> SRV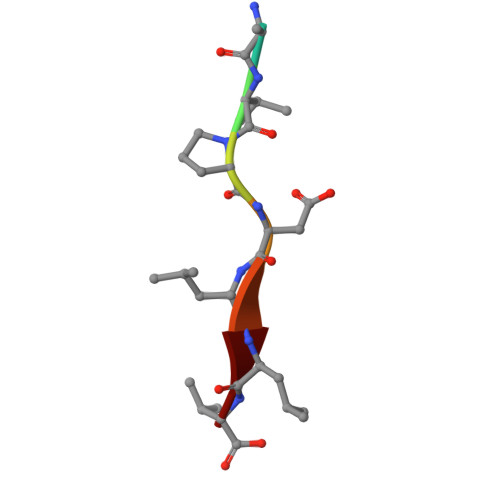PDLLV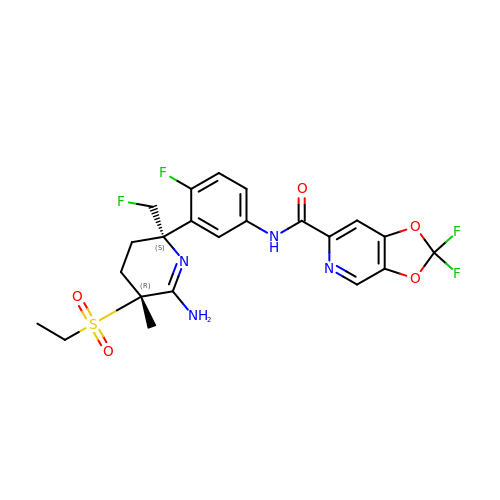N-{3-[(2S,5R)-6-amino-5-(ethanesulfonyl)-2-(fluoromethyl)-5-methyl-2,3,4,5-tetrahydropyridin-2-yl]-4-fluorophenyl}-2,2-difluoro-2H-[1,3]dioxolo[4,5-c]pyridine-6-carboxamide | C22 H22 F4 N4 O5 S | NDIQAOIHFVWZJQ-NHCUHLMSSA-N> ATGTVSLTDVGLDASYAGQVSIGTPAQDFLVIMDSGSSDLWVAGSTCTENFCKQTYTFDTSTSSSFITSSEAFNITYGSGDADGTLGTDTVSMAGFTVSDQTFGVVTSTSANLISYPLSGLMGLAWKSIASSGATPFWQTLAASGDWDSPEMGVYLKRYRGDNTASQIETDGGQILFGGLNTSLYNGSVNYISIDESEKDYWRIPLEAMVIQGNSVSIASSSGGSNPSCAIDTGTTLIGVP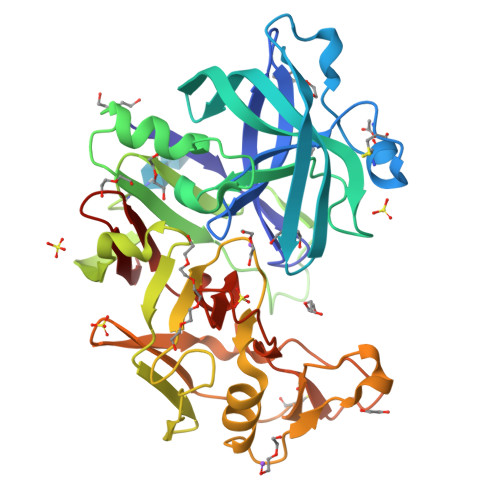SQTANRIYSQIAGAEALSASSGYEGYYQYPCDTEVTVSLQFGGMSYSISNADMNLGSFTRDTSMCTGAFFAMDMSSRSPVQWIVGASFIKNVYTAFRYNPAAIGFAELV> VVGGTEAQRNSWPSQISLQYRSGSSWAHTCGGTLIRQNWVMTAAHCVDRELTFRVVVGEHNLNQNDGTEQYVGVQKIVVHPYWNTDDVAAGYDIALLRLAQSVTLNSYVQLGVLPRAGTILANNSPCYITGW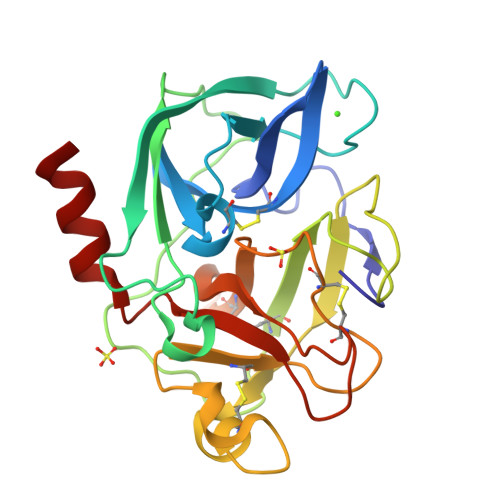GLTRTNGQLAQTLQQAYLPTVDYAICSSSSYWGSTVKNSMVCAGGDGVRSGCQGDSGGPLHCLVNGQYAVHGVTSFVSRLGCNVTRKPTVFTRVSAYISWINNVIASN>SGSVEDRVTQLERISNAHSQLLTQLQQQLSDNQSDIDSLRGQIQENQYQLNQVVER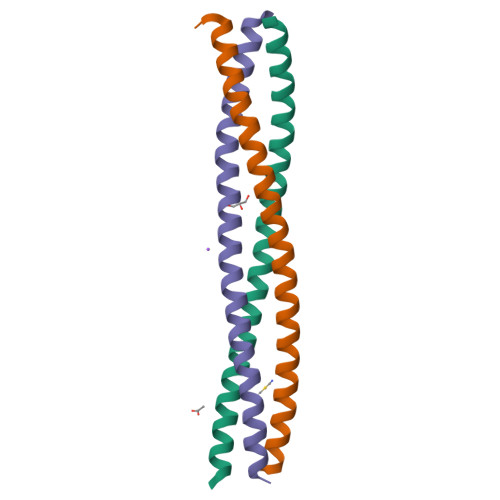QKQILLQIDSLSSGGAAAQ[6x]> MELRHLRYFVAVVEEQSFTKAADK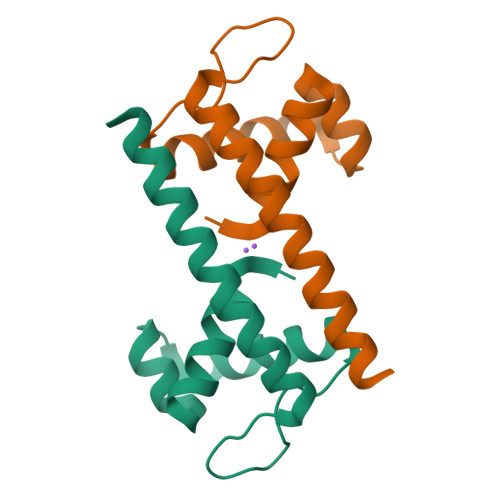LCIAQPPLSRQIQNLEEELGIQLLERGSRPVKTTPEGHFFYQYAIKLLSNVDQMVSMTKRIASGHHHHHH> MKIAIINMGNNVINFKTVPSSETIYLFKVISEMGLNVDIISLKNGVYTKSFDEVDVNDYDRLIVVNSSINFFGGKPNLAILSAQKFMAKYKSKIYYLFTAIRLPFSQSWPNVKNRPWAYLYTEEELLIKSPIKVISQGINLDIAKAAHKKVDNVIEFEYFPIEQYKIHMNDFQLSKPTKKTLDVIYGGSFRSGQRESKMVEFLFDTGLNIEFFGNAREKQFKNPKYPWTKAPVFTGKIPMNMVSEKNSQAIAALIIGDKNYNDNFITLRVWETMASDAVMLIDEEFDTKHRIINDARFYVNNRAELIDRVNELKHSDVLRKEMLSIQHDILNKTRAKK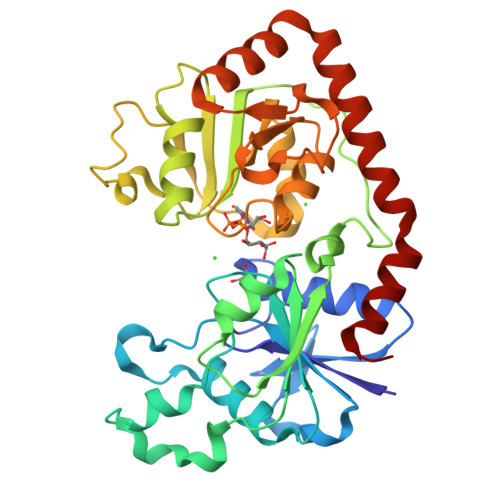AEWQDAFKKAIDL>AQDMVSPPPPIADEPLTVNTGIYLIECYSLDDKAETFKVNAFLSLSWKDRRLAFDPVRSGVRVKTYEPEAIWIPEIRFVNVENARDADVVDISVSPDGTVQYLERFSARVLSPLDFRRYPFDSQTLHIYLIVRSVDTRNIVLAVDLEKVGKNDDVFLTGWDIESFTAVVKPANFALEDRLESKLDYQLRISRMYFSYIPNIILPMLFILFISWTAFWSTSYEANVTLVVSTLIAHIAFNILVETNLPKTPYMTYTGAIIFMIYLFYFVAVIEVTVQHYLKVESQPARA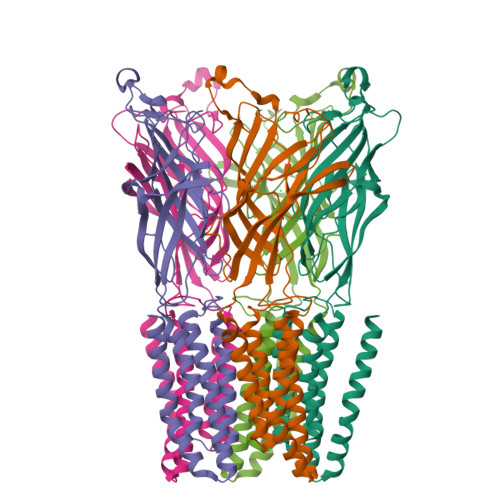ASITRASRIAFPVVFLLANIILAFLFFGF[5x]> GMAKATTIKDAIRIFEERKSVVATEAEKVELHGMIPPIEKMDATLSTLKACKHLALSTNNIEKISSLSGMENLRILSLGRNLIKKIENLDAVADTLEELWISYNQIASLSGIEKLVNLRVLYMSNNKITNWGEIDKLAALDKLEDLLLAGNPLYNDYKENNATSEYRIEVVKRLP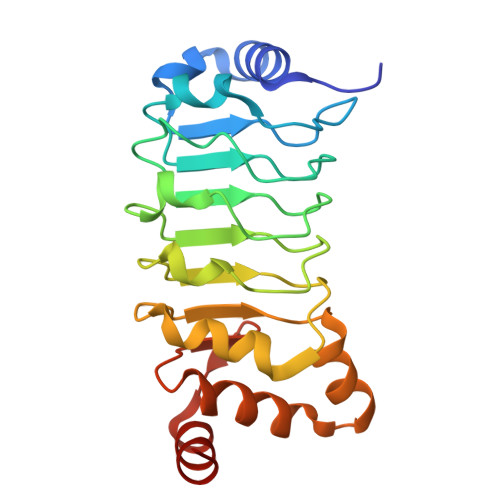NLKKLDGMPVDVDEREQANVARGG>[2x]GLSPEEKQRRAIASATEGGSVPQIRAPSHVPFLLIGGGTAAFAAARSIRARDPGARVLIVSEDPELPYMRPPLSKELWFSDDPNVTKTLQFRQWNGKERSIYFQPPSFYVSAQDLPNIENGGVAVLTGKKVVHLDVRGNMVKLNDGSQITFEKCLIATGGTPRSLSAIDRAGAEVKSRTTLFRKIGDFRALEKISREVKSITVIGGGFLGSELACALGRKSQASGIEVIQLFPEKGNMGKILPQYLSNWTMEKVKREGVKVMPNAIVQSVGVSGGRLLIKLKDGRKVETDHIVTAVGLEPNVE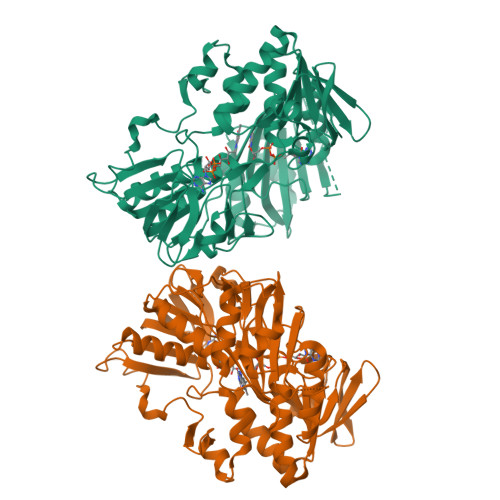LAKTGGLEIDSDFGGFRVNAELQARSNIWVAGDAACFYDIKLGRRRVEHHDHAVVSGRLAGENMTGAAKPYWHQSMFWSDLGPDVGYEAIGLVDSSLPTVGVFAKATAQDNPKSATEQSGTGIRSESETESEASEITIPPSAPAVPQVPVEGEDYGKGVIFYLRDKVVVGIVLWNVFNRMPIARKIIKDGEQHEDLNEVAKLFNIHED>GGVANASGASWGPPRGQYSAGAVAGLAAVVGFLIVFTVVGNVLVVIAVLTSRALRAPQNLFLVSLASADILVATLVMPFSLANELMAYWYFGQWWCGVYLALDVLFCTSSAVHLCAISLDRYWSVTQAVEYNLKRTPRRVKATIVAVWLISAVISFPPLVSLYRQPDGAAYPQCGLNDETWYILSSCIGSFFAPCLIMGLVYARIYRVAKLRTGIDCSFWNESYLTGSRDERKKSLLSKFGMDEGVTFMFIGRFDRGQKGVDVLLKAIEILSSKKEFQEMRFIIIGKGDPELEGWARSLEEKHGNVKVITEMLSREFVRELYGSVDFVIIPSYFEPFGLVALEAMCLGAIPIASAVGGLRDIITNETGILVKAGDPGELANAILKALELSRSDLSKFRENCKKRAMSFSVAQAREKRFTFVLAVVMGVWVLCWFPFFFSYSLYGICREACQVPGPLFKFFFWIGYCNSSLNPVIYTV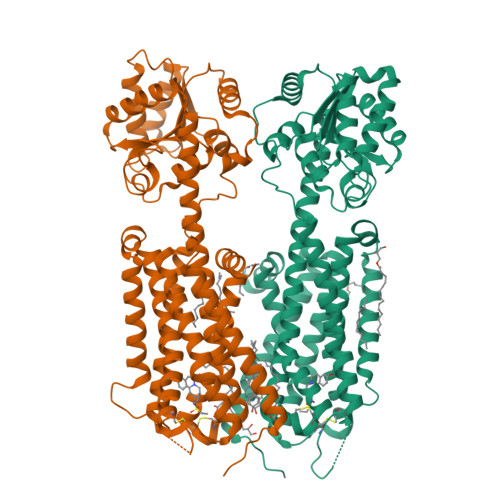FNQDFRRSFKHILFRRRRR[2x]> MAHAGRTGYDNREIVMKYIHYKLSQRGYEWDAGDDVEENRTEAPEGTESEVVHLTLRQAGDDFSRRYRRDFAEMSSQLHLTP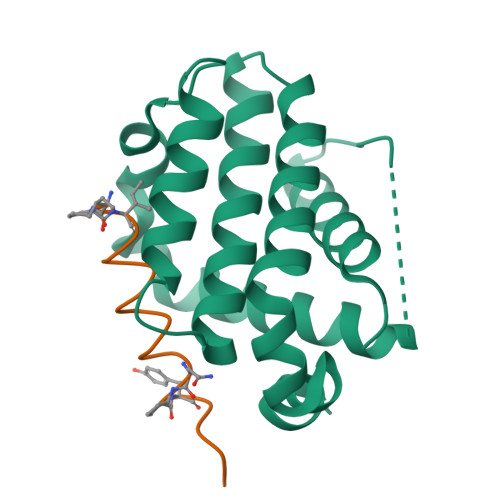FTARGRFATVVEELFRDGVNWGRIVAFFEFGGVMCVESVNREMSPLVDNIALWMTEYLNRHLHTWIQDNGGWDAFVELYGPSMR;> MAHAGRTGYDNREIVMKYIHYKLSQRGYEWDAGDDVEENRTEAPEGTESEVVHLTLRQAGDDFSRRYRRDFAEMSSQLHLTPFTARGRFATVVEELFRDGVNWGRIVAFFEFGGVMCVESVNREMSPLVDNIAIWMTEYLNRHLHTWIQDNGGWDAFVELYGPSMR> HHHHHHSSGENLYFQGHMRPERLTVRNFLGLKNVDIEFQSGITVVEGPNGAGKSSLFEAISFALFGNGIRYPNSYDYV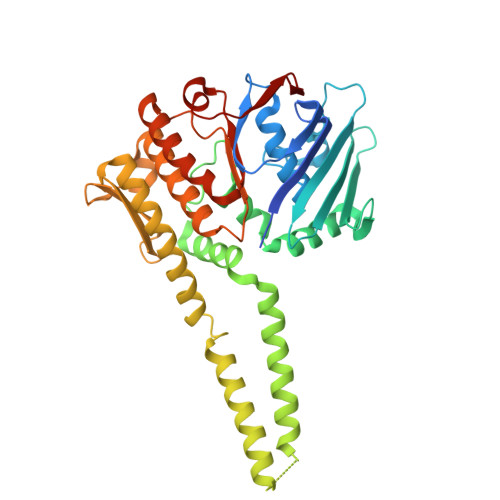NRNAVDGTARLVFQFERGGKRYEIIREINALQRKHNAKLSEILENGKKAAIAAKPTSVKQEVEKILGIEHRTFIRTVFLPQGEIDKLLISPPSEITEIISDVFQSKETLEKLEKLLKEKMKKLENEISSGGAGGAGGSLEKKLKEMSDEYNNLDLLRKYLFDKSNFSRYFTGRVLEAVLKRTKAYLDILTNGRFDIDFDDEKGGFIIKDWGIERPARGLSGGERALISISLAMSLAEVASGRLDAFFIDEGFSSLCTENKEKIASVLKELERLNKVIVFITCDREFSEAFDRKLRITGGVVVNE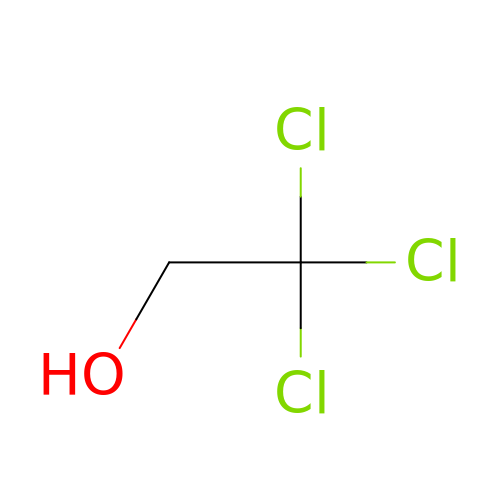2,2,2-tris-chloroethanol | C2 H3 Cl3 O | KPWDGTGXUYRARH-UHFFFAOYSA-N> GVYYATAYWMPTEKTIQVKNVLDRKGDAYGFYNNSVKTTGWGILEIKAGYGSQSLSNEIIMFAAGFLEGYLTAPHMDDHFTNLYPQLIKKRSMLNKVQDFLTKQDQWTRENIKYYKSDPFWRHADYVMAQMDGLFAGATKRAVLEGKKPMTLFQIQFLNAIGDLLDLIPS;> CSALIKVLPGFENIFFAHSSWYTYAAMLRIYKHWDFNIVDKDTSSSRLSFSSYPGFLESLDDFYLLSSGLVLLQTTNSVYNKTLLQHVVPQSLLAWQRVRVASMMAN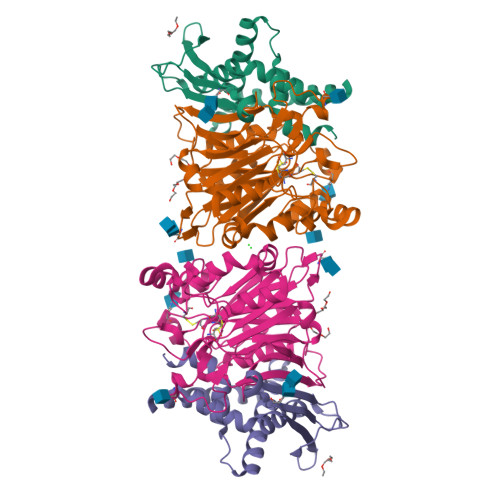NGKQWAEVFSKYNSGTYNNQYMVLDLKKVNLNHSLDEGTLYIVEQIPTYVEYSEQTAVLRRGYWPSYNIPFHEKVYNWSGYPILVKKLGLDYSYDLASRAKIFRRDQGKVTDMESMKYIMRYNNYKQDPYSKGDPCNTVCCREDLNSHSPSPGGCYDTKVADIYLASKYKAYAISGPTVQGGLPVFHWSRFNKTLHEGMPEAYNFDFITMKPIL> ASTSCNVVLTDSQGSFTSPCYPNDYPPSQSCNWTIQAPAGFIVQITFLDFELEEAQGCIYDRVVVKTGTSDAKFCGLTANGLTLNSTGNVMEVFFNSDFSVQKKGFHISYKQVAVTLRNQKVTMPKSSKTILRVSNSISIPVLTAFTVCFEIARTAQKATETIFTLSDAAGTSILAFEKTSNGMELFIGASYCSVDNFLTSSDITATMKPLCLTWTKSSGLIGVYFEGHYFSSICSASQIYTLQSGGLLQIAGKGSSSVSVDDQNLDGFIYNFRLWDHAMLSSELSALTCDTVGNVVDWDHSYWTIPGSSTQTDSTLSCSTAITTLSPGTAGCASGLGCPEDIFYRSTLVVTDEQTPDRDATAIISQWLNQTFQNWMYRVYVDGISLQLITVLSRITTTRQIYLALLVYKNTTDVNLAEVEIESMLRSAPAIGNGLTLDSVTVNLMENCQADEFPVHYRWPESRPTVTQYVPCFPYKDRNASRTCMINRDNYTSFWALPDRGNCTNITSITVSQENAMDVAVQLADISNNGLSKEELTQVVTKVMELVNIAKINATLASTVVTIISNVMVSSEDAQKDASETALKAVDELVQKIEFDGPSLTISSKNLVVGVSALDTTNFNGSTLSAFIATNTTDPQIDFD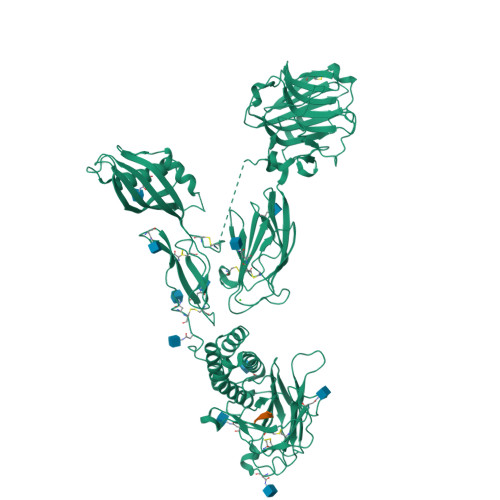SEAHNALAVVTLPPTLLQNLSLSQIEKVSRINFMFFGRTGLFQDHQNNGLTLNSYVVASSVGNFTIKNLQDPVRIEIAHLEYQKDPNPQCVFWDFNLQNYSGGWNSDGCKVGSDSNSNRTVCLCNHLTHFGILMDVSRAHHHHHHHH;> THFGILMDVSRA GraTA (Growth rate affecting Toxin–Antitoxin) is a type II TA module recently discovered in Pseudomonas putida. By sequence similarity, GraTA is most closely related to the higBA TA family. Here we show that GraA does not contain unstructured regions and forms a globular dimer while the toxin GraT contains an N-terminal intrinsically disordered region that is key for transcriptional regulation of the graTA operon as well as for the RNase activity of GraT. GraA binds tightly to the graTA operator and GraT prevents this interaction through steric interference from its N-terminal disordered region.

We determined the structure of the GraTA toxin–antitoxin complex at 2.2 Å resolution. With one His-tagged GraT monomer bound to each GraA monomer, a GraT-GraA2-GraT hetero-tetramer (hisGraT2A2 for short) is formed. Binding of GraT does not affect the structure of the GraA monomer but the relative orientation of each monomer in the GraA dimer is somewhat displaced. Upon binding of GraT, there is a 2.2° relative rotation of the GraA helix α3, which results in a 1.6 Å decrease of the distance between the HTH motifs. GraT binds on a negatively charged surface area of GraA, which is located opposite to the DNA binding surface. The contact surface area of one GraT monomer with GraA2 is 488 Å2. In GraT, residues S27, E30, R31, K32, A38, R43, D44, S47 and G50 are involved in hydrogen bonds with the GraA residues R7, E13, E18, D64, T66 and N72. In particular, A34, M35, A38, A39, P48 and P49 of GraT interact with a hydrophobic pocket on the surface of GraA formed by I9, I14, F19, M23, L63, F69 and L73. In GraT, on the other hand, the first 22 N-terminal residues together with the 6-His tag are located in an interstitial space and could not be traced due to lack of electron density. Instead, GraA inactivates GraT by inhibiting its binding to the ribosome due to steric hindrance via clashes between GraA and the ribosomal RNA as well as ribosomal protein S13.

>MLKNGMRPIHPGEILREEFQKEMGFSAAALARALGVATPTVNNILRERGGVSADMALRLSICLDTTPEFWLNLQTAFDLRTAEQQHGDEIIGSVQRLVA[2x];>MHHHHHHIRSFSCADTEALFTTGKTRRGSDIKSVAERKLAMLDAATELRDLRSPPGNRLESLSGNRADQHSIRVNDQWRLCFTWTEHGPVNVEIVDYH[2x]> MHHHHHHGKNHAGSPGCEESAAGKEKLPKMRLPTRSDMICGYACLKGTAAMRNTKRGSWYIEALAQVFSERACDM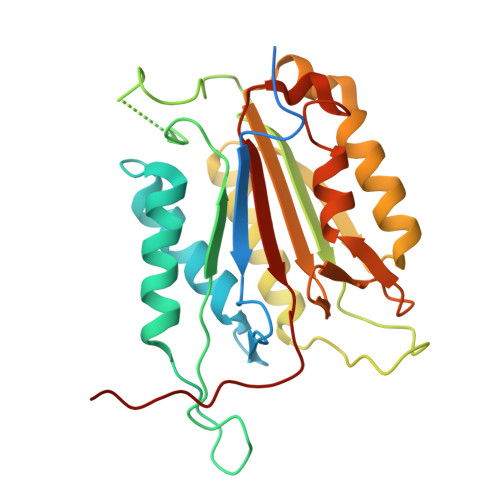HVADMLVKVNALIKDREGYAPGTEFHRCKEMSEYCSTLCRHLYLFPGGGVKPCTPEFYQTHFQLAYRLQSRPRGLALVLSNVHFTGEKELEFRSGGDVDHSTLVTLFKLLGYDVHVLCDQTAQEMQEKLQNFAQLPAHRVTDSCIVALLSHGVEGAIYGVDGKLLQLQEVFQLFDNANCPSLQNKPKMFFIQACRGDETDRGVDQQD> SPSAEECGYSDRVRSITLGNSTITTQECANVVVGYGVWPEYLKDNEATGEDQPTQPDVATCRFYTLESVQWMKNSAGWWWKLPDALSQMGLFGQNMQY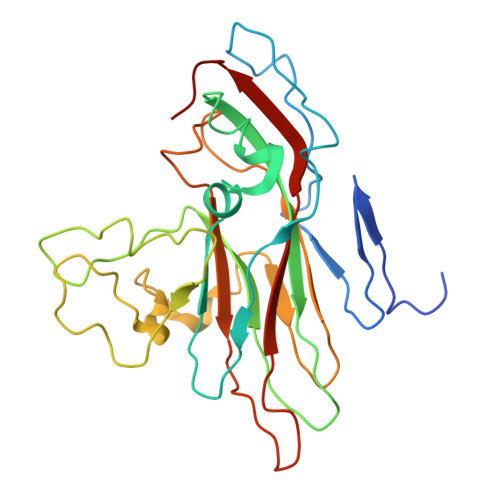HYLGRTGYTIHVQCNASKFHQGCLLVVCVPEAEMGCSNLNNTPKFAELSGGDNARMFTDTEVGTSNDKKVQTAVWNAGMGVGVGNLTIFPHQWINLRTNNSATIVMPYINSVPMDNMYRHNNLTLMIIPFVPLNYSEGSSPYVPITVTIAPMCAEYNGLRLASSQ>MIPVTEFRQFSEQQPAFRVLKPWWDVFTDYLSVAMLMIGVFGCTLQVMQDKIICLPKRVQPAQNHSSLSNVSQAVASTTPLPPPKPSPANPITVEMKGLKTDLDLQQYSFINQMCYERALHWYAKYFPYLVLIHTLVFMLCSNFWFKFPGSSSKIEHFISILGKCFDSPWTTRALSEVSGEDSDPKPAFSKMNGSMDKKSSTVSEDVEGSLVNSQSLKSIPEKFVVDKSTAGALDKKEGEQAKALFEKVKKFRLHVEEGDILYAMYVRQTVLKVIKFLIIIAYNSALVSKVQFTVDCNVDIQDMTGYKNFSCNHTMAHLFSKLSFCYLCFVSIYGLTCLYTLYWLFYRSLREYSFEYVRQETGIDDIPDVKNDFAFMLHMIDQYDPLYSKRFAVFLSEVSENKLKQLNLNNEWTPDKLRQKLQTNAHNRLELPLIMLSGLPDTVFEITELQSLKLEIIKNVMIPATIAQLDNLQELSLHQCSVKIHSAALSFLKENLKVLSVKFDDMRELPPWMYGLRNLEELYLVGSLSHDISRNVTLESLRDLKSLKILSIKSNVSKIPQAVVDVSSHLQKMCIHNDGTKLVMLNNLKKMTNLTELELVHCDLERIPHAVFSLLSLQELDLKENNLKSIEEIVSFQHLRKLTVLKLWHNSITYIPEHIKKLTSLERLSFSHNKIEVLPSHLFLCNKIRYLDLSYNDIRFIPPEIGVLQSLQYFSITCNVESLPDELYFCKKLKTLKIGKNSLSVLSPKIGNLLFLSYLDVKGNHFEILPPELGDCRALKRAGLVVEDALFETLPSDVREQMKTEENLYFQGAAAGDYKD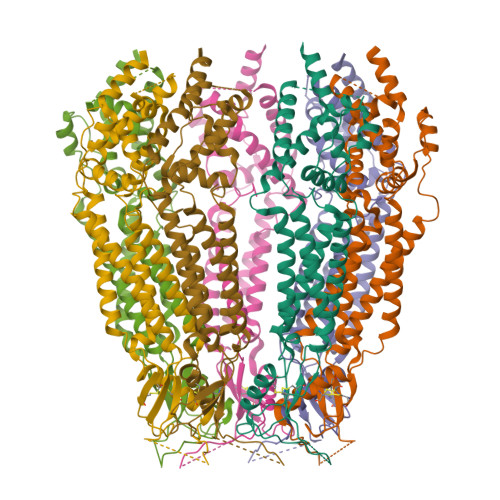DDDK[7x]> LADHVSVGETQIPKASTQHLLRKAGSLSAAGDTEVPIRGFVHMKLHKLVQ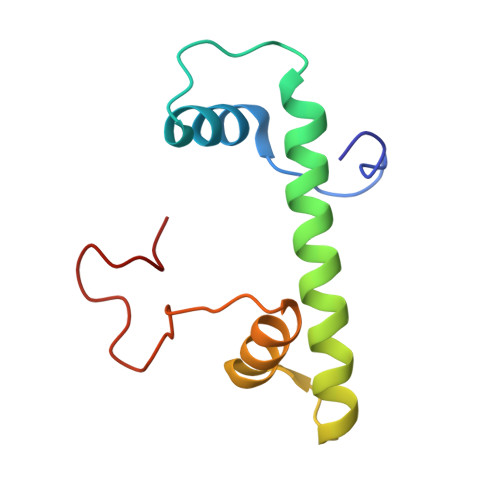KSLLAMQLAKRKTIMKSDVKKAAELMHLPVFAIPTKDSGAKGSVFLS>[2x]ADGKYAQKLFNDLFEDYSNALRPVEDTDKVLNVTLQITLSQIKDMDERNQILTAYLWIRQIWHDAYLTWDRDQYDGLDSIRIPSDLVWRPDIVLYNKADDESSEPVNTNVVLRYDG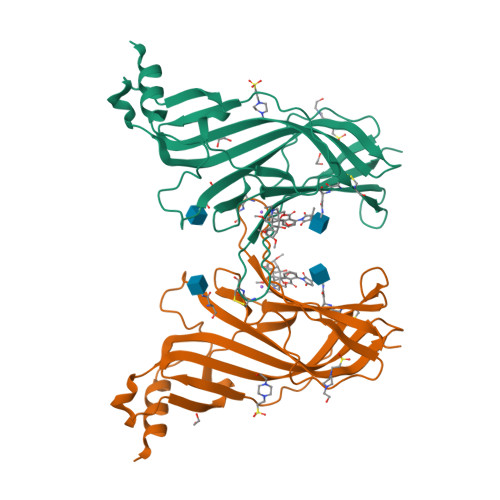LITWDAPAITKSSCVVDVTYFPFDNQQCNLTFGSWTYNGNQVDIFNALDSGDLSDFIEDVEWEVHGMPAVKNVISYGCCSEPYPDVTFTLLLKRRSHHHHHH>[12x]GAMAM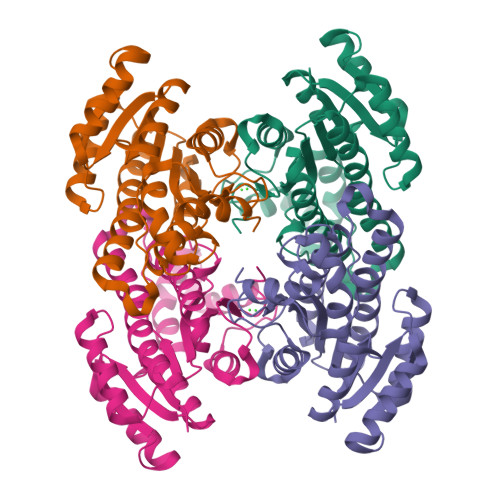EQVAVVIGGGQTLGAFLCEGLAQAGYHVAVADLNESNANRLADTINSRYGAGRAYGFKVDATDEASVEALARAVDETFGRADLLVYSAGVAKAAPITQFRLTDFDLSLQVNLVGYFLCSREFSKLMIRDGIKGRIIQINSKSGKVGSKHNSGYSAAKFGGVGLTQSLALDLAEYGITVHSLMLGNLLKSPMFQSLLPQYAEKLGITPEEVEPYYVDKVPLKRGCDYQDVLNVLLFYASDKAAYCTGQSINVTGGQVMF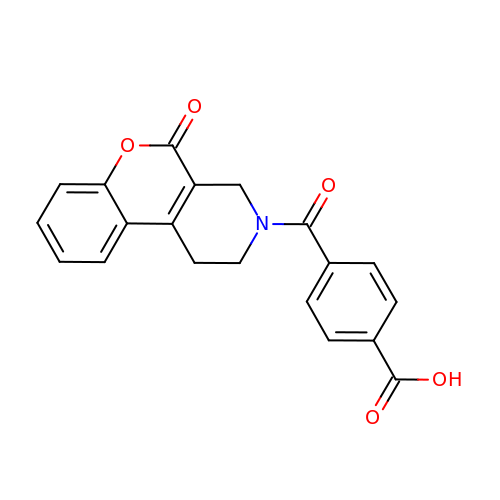4-(5-oxo-1,5-dihydro-2H-[1]benzopyrano[3,4-c]pyridine-3(4H)-carbonyl)benzoic acid | C20 H15 N O5 | OXUKTNZACAKVRG-UHFFFAOYSA-N> GMDETPIFKIKKLTIAENDRSEYIRYAEKNMHDSIPAEEGTLLIGSGHDDAHGEDNYEIEVFRNKGAEDLHIAGSHADDFVETVNKIATKQKVIDLHPEV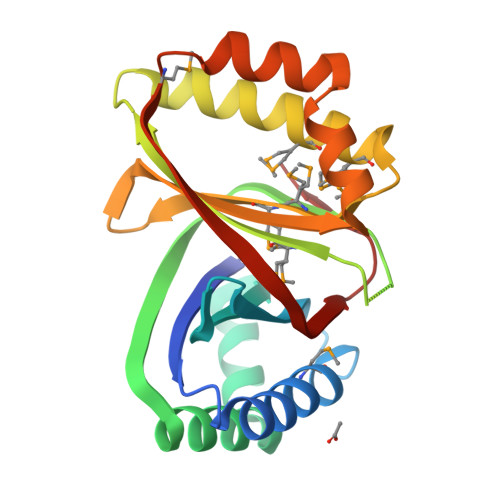ITTKAQRALNSYADNFVMRLIKVEVKDADAEKFSHAVKKEMTTSMASEPGMEIMMSGTNIDNPNEWYFIEVYANDEAYDIHVKTPHYKEYIEETDGMVKSRDVKTLVRDTLATQGAIVLD> MRLELPVIPLRNTVILPHTTTPVDVGRAKSKRAVEEAMGADRLIFLVAQRDPEVDDPAPDDLYTWGVQAVVKQAMRLPDGTLQVMVEARARAFQVTDYIPGPYLRARGEVFSEIFPIDEAVVRVLVEELKEAFEKYVANHKSLRLDRYQLEAVKGTSDPAMLADTIAYHATWTVAEKQEILELTDLEARLKKVLGLLSRDLERFELDKRVAQRVKEQMDTNQREYYLREQMKAIQKELGGEDGLSDLEALRKKIEEVGMPEAVKTKALKELDRLERMQQGSPEATVARTYLDWLTEVPWSKADPEVLDINHTRQVLDEDHYGLKDVKERILEYLAVRQLTQGLDVRNKAPILVLVGPPGVGKTSLGRSIARSMNRKFHRISLGGVRDEAEIRGHRRTYIGAMPGKLIHAMKQVGVINPVILLDEIDKMSSDWRGDPASAMLEVLDPEQNNTFTDHYLDVPYDLSKVFFITTANTLQTIPRPLLDRMEVIEIPGYTNMEKQAIARQYLWPKQVRESGMEGRIEVTDAAILRVISEYTREAGVRGLERELGKIARKGAKFWLEGAWEGLRTIDASDIPTYLGIPRYRPDKAETEPQVGTAQGLAWTPVGGTLLTIEVAAVPGSGKLSLTGQLGEVMKESAQAALTYLRAHTQDYGLPEDFYNKVDLHVHVPDGATPKDGPSAGITMATAIASALSRRPARMDIAMTGEVSLRGKVMPIGGVKEKLLAAHQAGIHKIVLPKDNEAQLEELPKEVLEGLEIK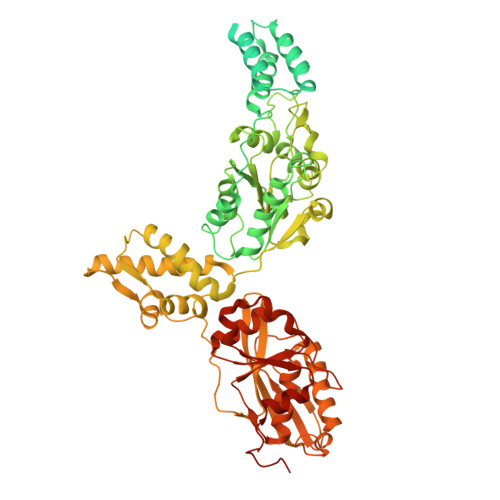LVEDVGEVLEYLLLPEPTMPPVVQPSDNRQQPGAGA> SVTIDHTTENAAPAQAPVSDRAWALFRALDGKGLVPDGYVEGWKKTFEEDFSPRRGAELVARAWTDPEFRQLLLTDGTAAVAQYGYLGPQGEYIVAVEDTPTLKNVIVCSLCSCTAWPILGLPPTWYKSFEYRARVVREPRKVLSEMGTEIAS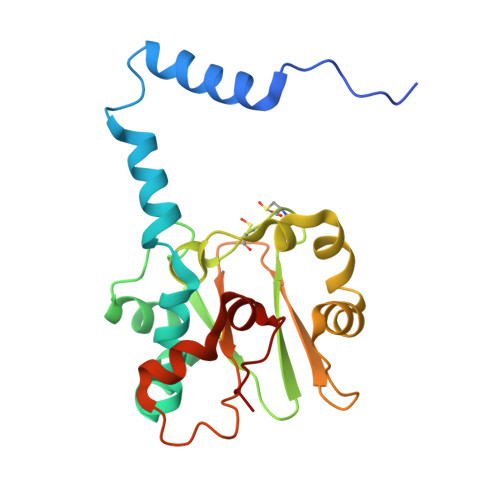DIEIRVYDTTAETRYMVLPQRPAGTEGWSQEQLQEIVTKDCLIGVAIPQVPTV> DSYTHLSFYEKRELFRKKLREIEGPEVTLVNEVDDEPCPSLDFQFISQYRLTQGVIPPDPNAQSGCNCSSLGGCDLNNPSRCECLDDLDEPTHFAYDAQGRVRADTGAVIYECNSACSCSMECPNRVVQRGRTLPLEIFKTKEKGWGVRSLRFAPAGTFITCYLGEVITSAEAAKRDKNYDDDGITYLFDLDMFDDASEYTVDAQNYGDVSRFFNHSCSPNIAIYSAVRNHGARTIYDLAFFAIKDIQPLEELTFDYAGAKDFSPVQSQKSQQNRISKLRRQCKCGSANCRGWLFG;> SYTHLSFYEKRELFRKKLREIEGPEVTLVNEVDDEPCPSLDFQFISQYRLTQGVIPPDPNAQSGCNCSSLGGCDLNNPSRCECLDDLDEPTHFAYDAQGRVRADTGAVIYECNSACSCSMECPNRVVQRGRTLPLEIFKTKEKGWGVRSLRFAPAGTFITCYLGEVITSAEAAKRDKNYDDDGITYLFDLDMFDDASEYTVDAQNYGDVSRFFNHSCSPNIAIYSAVRNHGARTIYDLAFFAIKDIQPLEELTFDYAGAKDFSPVQSQKSQQNRISKLRRQCKCGSANCRGWLF

Clr4 is the sole H3K9me2/3 methyltransferase in the fission yeast Schizosaccharomyces pombe, and recent evidence suggests that ubiquitination of lysine 14 on histone H3 (H3K14ub) plays a key role in H3K9 methylation. The SUV39 enzymatic activity facilitates the transfer of a methyl group from S-adenosyl-L-methionine (SAM) to the ε-amino group of lysine 9 on histone H3 with high specificity, thereby converting the cofactor to S-adenosyl-L-homocysteine (SAH). Our structure-function approach shows that the H3K14ub substrate binds specifically and tightly to the catalytic domain of Clr4, and thereby stimulates the enzyme by over 250-fold. We combined biochemical and structural methods to decipher the molecular mechanism governing the stimulation of Clr4 by H3K14ub. These experiments identified a ubiquitin binding region (UBR) in the catalytic domain of Clr4, which mediates H3K14ub binding, and mutations that disrupt this interaction interface lose heterochromatin function.

Based on the Clr4 structure and sequence conservation, we further chose to mutate three phenylalanines that intersect orthogonally with the GS253 mutations on the surface of Clr4 (F256A, F310A, and F427A, referred to as Clr4-3FA). The Clr4-3FA mutant showed very stable biochemical behavior and crystallized readily. To determine the effect of the 3FA mutations on the folding of Clr4, we solved the structure by X-ray crystallography. These efforts resulted in a 2.46 Å structure of Clr4-3FA. When comparing with previous X-ray structures of Clr4, we observed no significant difference in global or local protein folding between the wild-type Clr4 KMT domains and the Clr4-3FA mutant (RMSD = 0.37 Å). This indicates that the Clr4-3FA mutations do not induce significant structural changes. In contrast, Clr4-GS253 and Clr4-3FA showed complete loss of binding to H3K14ub under the same conditions. Comparison of the specificity constants ksp shows that the efficiency of the UBR mutants on H3K14ub drops approximately 27-fold for Clr4-3FA and 48-fold for Clr4-GS253 compared to the wild-type. In contrast to the enzymatic activity on H3K14ub, the activity on unmodified H3 peptides is only mildly affected resulting in a ksp, that is, 91% of wild-type for Clr4-3FA and 78% for Clr4-GS253. The model suggests that F310, which is also mutated in Clr4-3FA, is unlikely to be involved directly in the interaction with ubiquitin as the N-terminal residues 253–256 shield F310 from interacting with ubiquitin.> 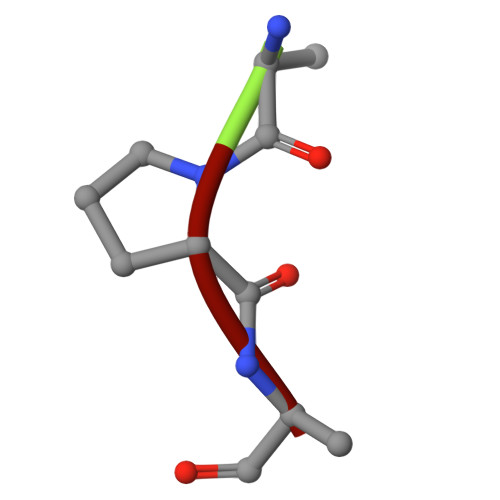APA> MSDSIQRTSVGDFPISQTVTVPASASLIFISGTLPDLADPHAPAGTPAAYGNTQVQTVSVFNKLRRILQQQDLDLGDIVQLRVFLV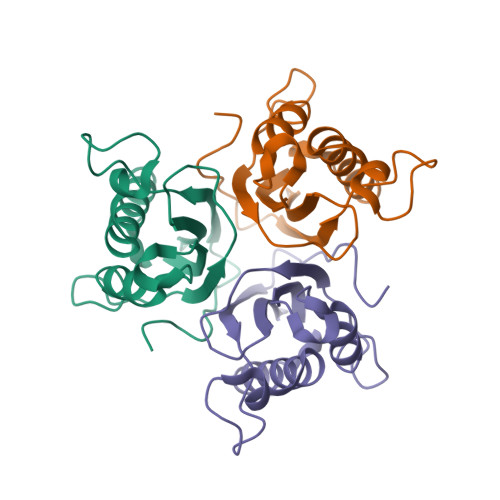GAEETGGKLDFAGLQAGYTQFFGTPEQPLKPARTALQVVALPLPGALIEVEAVAARSA>[2x]SNMVKIVTVKTQAYQDQKPGTSGLRKRVKVFQSSANYAENFIQSIISTVEPAQRQEATLVVGGDGRFYMKEAIQLIARIAAANGIGRLVIGQNGILSTPAVSCIIRKIKAIGGIILTASHNPGGPNGDFGIKFNISNGGPAPEAITDKIFQISKTIEEYAVCPDLKVDLGVLGKQQFDLENKFKPFTVEIVDSVEAYATMLRSIFDFSALKELLSGPNRLKIRIDAMHGVVGPYVKKILCEELGAPANSAVNCVPLEDFGGHHPDPNLTYAADLVETMKSGEHDFGAAFDGDGDRNMILGKHGFFVNPSDSVAVIAA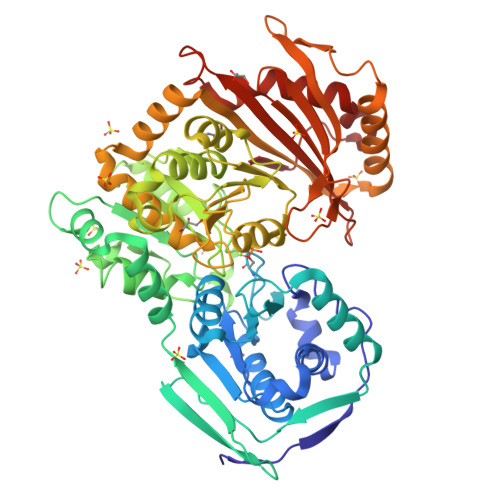NIFSIPYFQQTGVRGFARSMPTSGALDRVASATKIALYETPTGWKFFGNLMDASKLSLCGEESFGTGSDHIREKDGLWAVLAWLSILATRKQSVEDILKDHWQKYGRNFFTRYDYEEVEAEGANKMMKDLEALMFDRSFVGKQFSANDKVYTVEKADNFEYSDPVDGSISRNQGLRLIFTDGSRIVFQLSGTGSAGATIRLYIDSYEKDVAKINQDPQVMLAPLISIALKVSQLQERTGRTAPTVIT> GMKQPNYYQDVKQFHQTFHHPGADQPTAIPLDRGVKRATWTAEEAVVEFLHQSSQNETEFLAAIETFKAGL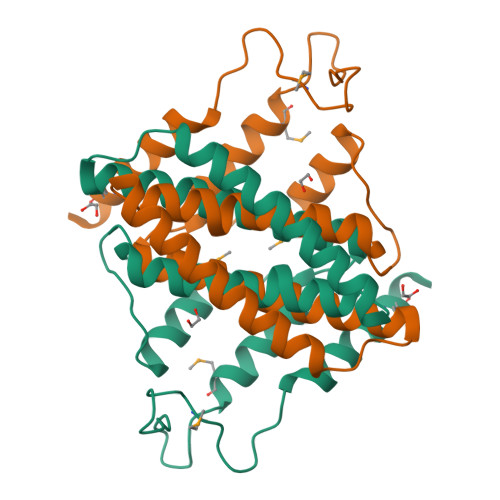DQAVKKSLKETYPVTEVERLVGQGDALTDALYFIMGSFVEAGLEPGPLFEIVQQANMAKLGPDGQPIFRESDQKVMKPDGWLPPEPQLEAEVVRQMKEKA> GSHMSQSNRELVVDFLSYKLSQKGYSWSQFSDVEENRTEAPEGTESEMETPSAINGNPSWHLADSPAVNGATGHSSSLDAREVIPMAAVKQALREAGDEFELRYRR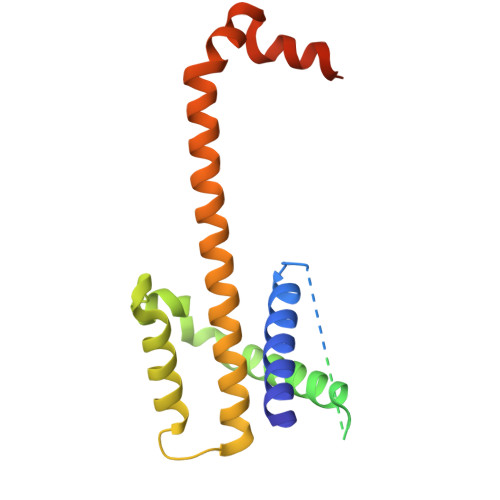AFSDLTSQLHITPGTAYQSFEQVVNELFRDGVNWGRIVAFFSFGGALCVESVDKEMQVLVSRIAAWMATYLNDHLEPWIQENGGWDTFVELYGNNAAAESRKGQER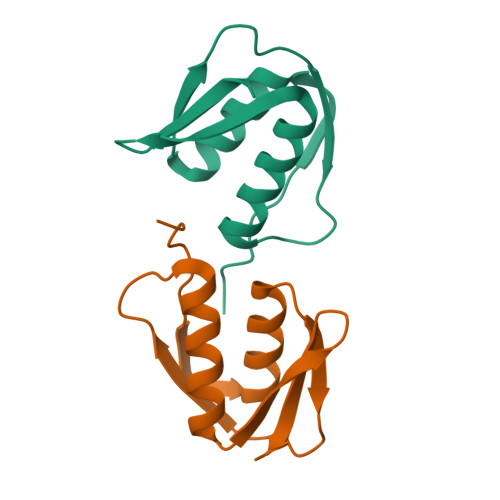>GAMATFTANFKDTDLKSFIETVGANLNKTIIMGPGVQGKVSIRTMTPLNERQYYQLFLNLLEAQGYAVVPMENDVLKVVKS[2x]> SNAMAGTLDLDKGCTVEELLRGCIEAFDDSGKVRDPQLVRMFLMMHPWYIPSSQLAAKLLHIYQQSRKDNSNSLQVKTCHLVRYWISAFPAEFDLNPELAEQIKELKALLDQEGNRRHSSLIDIDSVPTYKWKRQVTQRNPVGQKKRKMSLLFDHLEPMELAEHLTYLEYRSFCKILF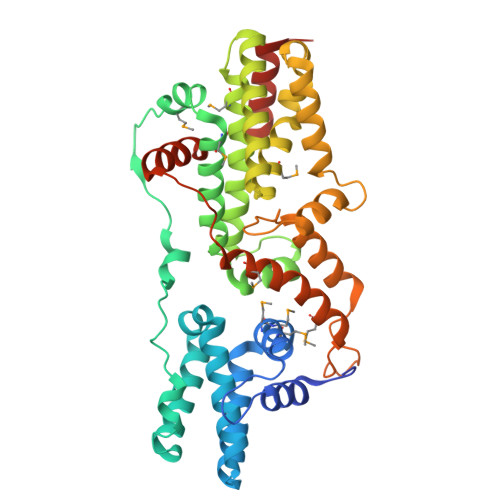QDYHSFVTHGCTVDNPVLERFISLFNSVSQWVQLMILSKPTAPQRALVITHFVHVAEKLLQLQNFNTLMAVVGGLSHSSISRLKETHSHVSPETIKLWEGLTELVTATGNYGNYRRRLAACVGFRFPILGVHLKDLVALQLALPDWLDPARTRLNGAKMKQLFSILEELAMVTSLRPPVQANPDLLSLLTVSLDQYQTEDELYQLSLQREPRSKSSPTS A HEPN (higher eukaryote and prokaryote nucleotide binding) nuclease Las1 and a polynucleotide kinase Grc3 assemble into a tetramerase responsible for rRNA maturation. Las1 and Grc3 are highly conserved proteins and have recently been identified as core enzymes involved in processing and removing ITS2 spacer, which is a key step in the synthesis of 60S ribosomal subunit. Recent studies have demonstrated that Las1 is an endoribonuclease that contains a HEPN (higher eukaryote and prokaryote nucleotide binding) domain responsible for rRNA processing. Grc3 is a polynucleotide kinase responsible not only for Las1 nuclease activation, but also for nonspecific phosphorylation of the 5′-OH of the 26S pre-rRNA produced by Las1 cleavage, providing a signal for further processing by Rat1-Rai1 exonuclease.

To elucidate how Las1 and Grc3 cooperate to direct ITS2 cleavage and phosphorylation, we determined the cryo-EM and crystal structures of full-length ScLas1-Grc3 complex at 3.07 Å and 3.69 Å resolution, respectively. Since the crystal structures have similar quality and resolve more structural information than the cryo-EM structures, the subsequent presentations and descriptions are based more on the crystal structures. The ScLas1-Grc3 tetramer structure shows that two Grc3 GCT are stabilized by two HEPN domains of Las1. Each Grc3 GCT binds to a groove in each Las1 HEPN domain and extends to the ribonuclease active center, which is formed by the two HEPN domains via dimerization. Both the crystal and cryo-EM structures show that the conserved catalytic residues Arg129, His130, His134 with two copies from two HEPN domains form a symmetric catalytic active pocket. Specifically, the side chain of Trp617 within Grc3 GCT inserts into the active pocket and forms packing and hydrogen bond with catalytic residue His134. Moreover, Trp617 and His615 in Grc3 form extensive hydrogen bond with residues Arg136, Leu99, Gly98, and His54 within Las1. Our crystal and cryo-EM structures exhibit that the Las1 LCT is located in a groove in the CTD domain of Grc3. The side chains of Trp488, Trp494, and Phe499 of Las1 LCT are inserted into the three hydrophobic core regions of Grc3 CTD and form stable hydrophobic interactions with multiple hydrophobic residues of Grc3. Notably, compared with CjGrc3-bound CjLas1, ScGrc3-bound ScLas1 has a more compact catalytic pocket, which may explain why ScLas1 shows better ITS2 cleavage activity than CjLas1 in the presence of Grc3.

>[3x]MVIDSKQDLPQYTKDSGSESDSDSSNNFIVESPSIPSSKSATVVLNSEEYEDDEGDDLNGLDAELIDNITYEGDEDETMFVGLKEKQKLHLSGVFRLQVVKGGIVYNNVHYNASREILTFWHPLSQSIPTIDFSHFAGWQDTFFMPRNNRFKIRDEEFKSFPCVLRVFNSNHTGLLEAGHLYRDVNYLWKPKEPYFPLNERTTYHLLHESDRIQSLSVPGYWSTPLEKLYLSHKNAAYDTRIMVIGGKNSGKSTFLRLLLEKFTQDIRDSTTSQEELVYLDLDPGQPEYSLPDSISLNKILSSPISLGQHLCQGSNFQTLLQFYAGSSSPQDEPTSYLNCADKLIDHLEEQAFFGTSLLNLPGWIKGFGMQILNHIIRKYKPTHLLFLETANSKRHLDELTIPQSFSTSLRDAYAPEVVRVPAHSLNHTLSSRFHASQLRTFKILALFHKITQFDYDFAPLLKSAPLQISYGKGKSGIKGIQFPMEFQDLNPQDIKSALEGTVIGIYTYSGEDSLEVKSLNTFPILQSCTSSSKNFITLGLIHSIDTSQQIMNIYVPPCHTQILDKQPEDAQWIIVRNKTETPFCDFLPSPRTITWDDNIQIPFATFERRKKLEHVWKVRKNVMRRGQFMKR;>MIPPRIVPWRDFAELEELKLWFYPKSKGTIEDKRQRAVQRVQSYRLKGSQYLPHVVDSTAQITCAVLLDEKEACLGVHQDSIPIRLSYVMALIRFVNGLLDPTQQSQFAIPLHTLAAKIGLPSWFVDLRHWGTHERDLPGLEMLRWAANEALSWLYDHYWNDEELEDDRDDDDDDDDTGYGYRRNDKLEKYMESLTKTLDKWKRLRNEFLEYKWVWENANDSLITSSNFSGDNLVNYDAEKRKSSHASSSETMIRENLRQWQELWKLSIYHNVVLEKFFNNYDPLLLKVLMLNLNNFDWKVIEWVARNYRTQQDDSNITTILKRKFNAWKELQKRLLDVIINNLNNKNFKNKWQNWEKLIDENASYLILYFCQSMLAKLETEKITGNSWRNKKRRKQIDSTVEIEAKLKENIDNLSLRFNEGEIKLYDFIPAEKDSVPLKKEVSPALKADTNDILGDLASLKQRMSSFGTVGKKNKQEENRATPVKNWSRVQNWKPKPFGVL[3x]CA forms the capsid shell surrounding the viral core that protects and transports the viral genome and also interacts with host cell factors that are necessary for trafficking, nuclear entry and proviral integration. Further, we assemble particles from HML2 CArec in vitro and use single-particle cryogenic electron microscopy (cryo-EM) to determine the high-resolution structures of four different types of Fullerene shell assemblies. Our studies of HML2 CArec show that an ERV retains the ability to form capsid assemblies using the same architecture as exogenous viruses. Analysis of the shell structures reveals the intra- and inter-molecular interactions that drives CA assembly into pentamers and hexamers and their association into shells that encapsidate the retroviral genome.

The majority species comprises 12 HML2 CArec pentamers with all interfaces equivalent, obeying perfect T = 1 icosahedral symmetry. The structure is resolved at the highest resolution (2.7 Å), likely corresponding to the 32S species observed in sedimentation experiments. The NTDs of each pentamer are associated proximal to the five-fold axis and form a layer of structure at a radius of 86.3 Å (NTD centroid distance) from the particle centre. Beneath the NTDs, the CTDs form an “inner cage” layer at a radius of 64.7 Å (CTD centroid distance), and more distal to the five-fold axis. The NTD layer does not contribute to inter-pentamer interactions and so the entire inter-pentamer interface is mediated through inner cage CTD–CTD interactions across icosahedral two-fold axes. In HML2, the vertical displacement between the NTD and CTD, as judged by the centre of mass (CoM) of the two layers, is 21.6 Å. In the pentamer, residue R143 located at the C terminus of α6 in the NTD makes a hydrogen bond to the main-chain carbonyl of K182, located at the C terminus of α7 in the CTD. This configuration facilitates formation of a specific hydrogen bonding arrangement between CTD residues D171 on α7 and K229 on α10 with S79′ and D90′ on α4 of the neighbouring monomer NTD (′ denoting a neighbouring monomer) and defines the pentamer conformation. By comparison, at the unique type of CTD–CTD interface in the T = 1 particle the α8 centroid displacement is maintained at 12 Å, but the crossing angle is significantly enlarged to 65°. This has the effect of twisting the interface relative to the solution state to meet the constraint imposed by icosahedral particle geometry, although remarkably, the hydrophobic interactions of A189, V192 and I193 are preserved, and although much of the polar network is lost, a new compensatory S157–E200–N159 interaction contact is present.

> PVTLEPMPPGEGAQEGEPPTVEARYKSFSIKMLKDMKEGVKQYGPNSPYMRTLLDSIAHGHRLIPYDWEILAKSSLSPSQFLQFKTWWIDGVQEQVRRNRAANPPVNIDADQLLGIGQNWSTISQQALMQNEAIEQVRAICLRAWEKIQDPGSACPSFNTVRQGSKEPYPDFVARLQDVAQKSIADEKARKVIVELMAYENANPECQSAIKPLKGKVPAGSDVISEYVKACDGIGGAMHKAMLMAQLE>AEGTRGRSSTARCSLFGSDFVNTFDGSMYSFAGYCSYLLAGGCQKRSFSIIGDFQNGKRVSLSVYLGEFFDIHLFVNGTVTQGDQRVSMPYASKGLYLETEAGYYKLSGEAYGFVARIDGSGNFQVLLSDRYFNKTCGLCGNFNIFAEDDFMTQEGTLTSDPYDFANSWALSSGEQWCERASPPSS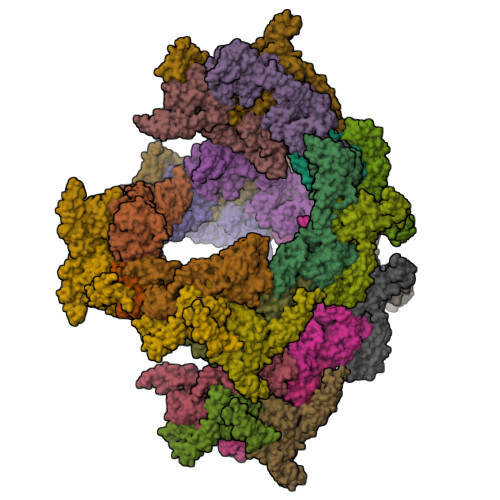SCNISSGEMQKGLWEQCQLLKSTSVFARCHPLVDPEPFVALCEKTLCECAGGLECACPALLEYARTCAQEGMVLYGWTDHSACSPVCPAGMEYRQCVSPCARTCQSLHINEMCQERCVDGCSCPEGQLLDEGLCVESTECPCVHSGKRYPPGTSLSRDCNTCICRNSQWICSNEECPGECLVTGQSHFKSFDNRYFTFSGICQYLLARDCQDHSFSIVIETVQCADDRDAVCTRSVTVRLPGLHNSLVKLKHGAGVAMDGQDVQLPLLKGDLRIQHTVTASVRLSYGEDLQMDWDGRGRLLVKLSPVYAGKTCGLCGNYNGNQGDDFLTPSGLAEPRVEDFGNAWKLHGDCQDLQKQHSDPCALNPRMTRFSEEACAVLTSPTFEACHRAVSPLPYLRNCRYDVCSCSDGRECLCGALASYAAACAGRGVRVAWREPGRCELNCPKGQVYLQCGTPCNLTCRSLSYPDEECNEACLEGCFCPPGLYMDERGDCVPKAQCPCYYDGEIFQPEDIFSDHHTMCYCEDGFMHCTMSGVPGSLLPDAVLSSPLSHRSKR[14x];>[14x]SLSCRPPMVKLVCPADNLRAEGLECTKTCQNYDLECMSMGCVSGCLCPPGMVRHENRCVALERCPCFHQGKEYAPGETVKIGCNTCVCQDRKWNCTDHVCDATCSTIGMAHYLTFDGLKYLFPGECQYVLVQDYCGSNPGTFRILVGNKGCSHPSVKCKKRVTILVEGGEIELFDGEVNVKRPMKDETHFEVVESGRYIILLLGKALSVVWDRHLSISVVLKQTYQEKVCGLCGNFDGIQNNDLTSSNLQVEEDPVDFGNSWKVSSQCADTRKVPLDSSPATCHNNIMKQTMVDSSCRILTSDVFQDCNKLVDPEPYLDVCIYDTCSCESIGDCACFCDTIAAYAHVCAQHGKVVTWRTATLCPQSCEERNLRENGYECEWRYNSCAPACQVTCQHPEPLACPVQCVEGCHAHCPPGKILDELLQTCVDPEDCPVCEVAGRRFASGKKVTLNPSDPEHCQICHCDVVNLTCEACQEPGGLVVPPHHHHHH[(2~{R},3~{S},4~{S})-2,3,4,5-tetrakis(oxidanyl)pentyl] 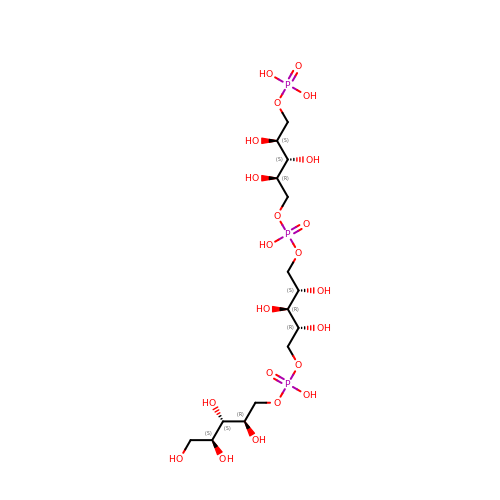[(2~{R},3~{R},4~{S})-2,3,4-tris(oxidanyl)-5-[oxidanyl-[(2~{R},3~{S},4~{S})-2,3,4-tris(oxidanyl)-5-phosphonooxy-pentoxy]phosphoryl]oxy-pentyl] hydrogen phosphate | C15 H35 O22 P3 | OFDIUZNQYOUSRP-VACZDDTMSA-N>[2x]MTVGTLVASVLPATVFEDLAYAELYSDPPGLTPLPEEAPLIARSVAKRRNEFITVRHCARIALDQLGVPPAPILKGDKGEPCWPDGMVGSLT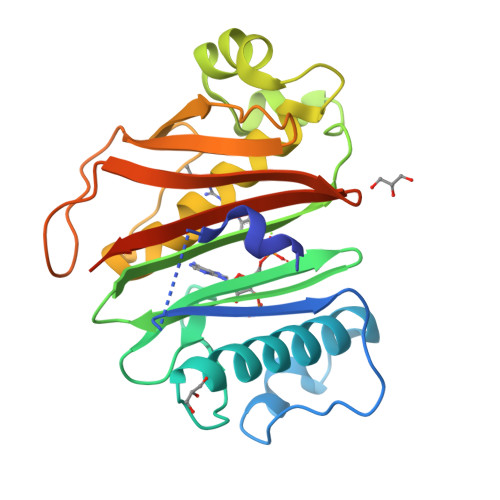HCAGYRGAVVGRRDAVRSVGIDAEPHDVLPNGVLDAISLPAERADMPRTMPAALHWDRILFCAKEATYKAWFPLTKRWLGFEDAHITFETDSTGWTGRFVSRILIDGSTLSGPPLTTLRGRWSVERGLVLTAIVLAGENLYFQSAGHHHHHH> MKKVEAIIRPEKLEIVKKALSD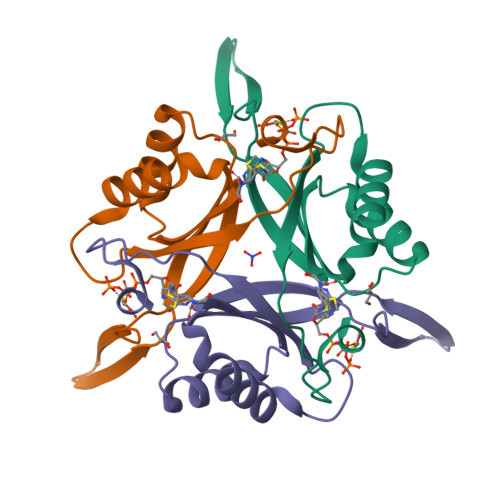AGYVGMTVSEVKGRGVQGGIVERYRGREYIVDLIPKVKIELVVKEEDVDNVIDIICENARTGNPGDGKIFVIPVERVVRVRTKEEGKEAL>[3x]GSHMASPNGQTKPLPALKLALEYIVPCMNKHGICVVDDFLGKETGQQIGDEVRALHDTGKFTDGQLVSQKSDSSKDI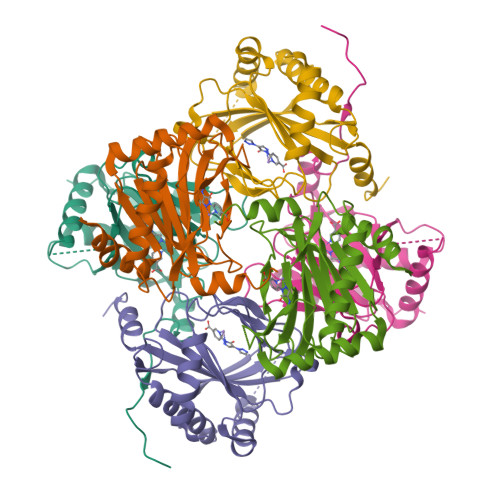RGDKITWIEGKEPGCETIGLLMSSMDDLIRHCNGKLGSYKINGRTKAMVACYPGNGTGYVRHVDNPNGDGRCVTCIYYLNKDWDAKVSGGILRIFPEGKAQFADIEPKFDRLLFFWSDRRNPHEVQPAYATRYAITVWYFDADERARAKVKYLTGEKGVRVELNKPSDSVGKDVF6-[(3-Chloro-6,7,10,11-tetrahydro-9-methyl-7,11-methanocycloocta[b]quinolin-12-yl)amino]-N-(4-hydroxy-3-methoxybenzyl)hexanamide | C31 H36 Cl N3 O3 | 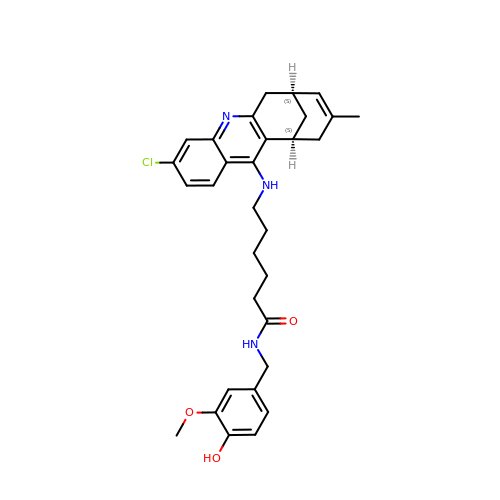AUFZKQKTTGOKEM-FCHUYYIVSA-N> GSALSEIETRHSEI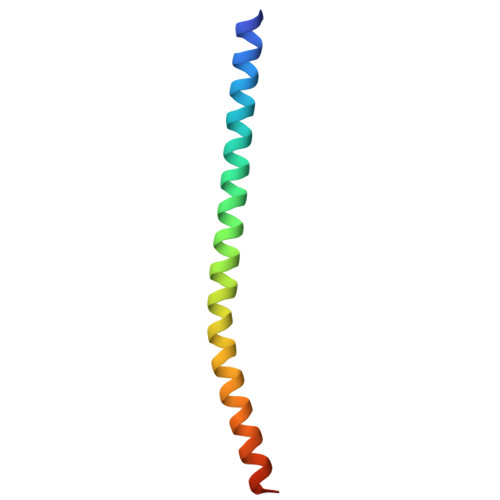IKLENSIRELHDMFMDMAMLVESQGEMIDRIEYNVEHAVDYVERAVSDTKK3-[(3~{R})-3-[aminocarbonyl(oxidanyl)amino]but-1-ynyl]-~{N}-[(3~{S})-3-phenyl-3-[4-(trifluoromethyloxy)phenyl]propyl]benzamide | C28 H26 F3 N3 O4 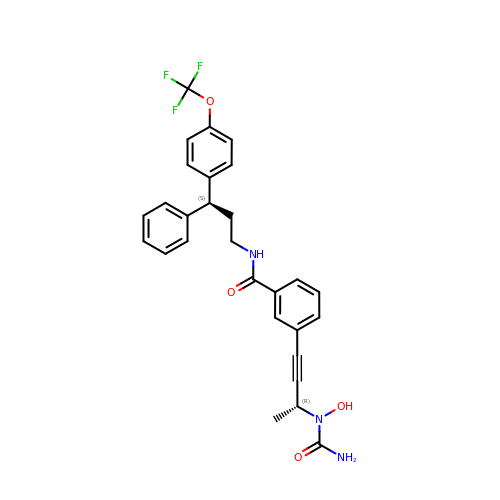| HQXPQGGUDYBGKG-CLOONOSVSA-N> MSEFRIHHDVNELLSLLRVHGGDGAEVYIDLLQKNRTPYVTTTVSAHSAKVKIAEFSRTPEDFLKKYDELKSKNTRNLDPLVYLLSKLTEDKETLQYLQQNAKERAELAAAAVGSSTTSINVPAAASKISMQELEELRKQLGSVATGSTLQQSLELKRKMLRDKQNKKNSGQHLPIFPAWVYERPALIGDFLIGAGISTDTALPIVLLRWNLALSPRLKCSGVISAHCNLHLPGTLPLASQESAVVEDLLYVLVGVDGRYVSAQPLAGRQSRTFLVDPNLDLSIRELVHRILPVAASYSAVTRFIEEKSSFEYGQVNHALAAAMRTLVKEHLILVSQLEQLHRQGLLSLQKLWFYIQPAMRTMDILASLATSVDKGECLGGSTLSLLHDRSFSYTGDSQAQELCLYLTKAASAPYFEVLEKWIYRGIIHDPYSEFMVEEHELRKERIQED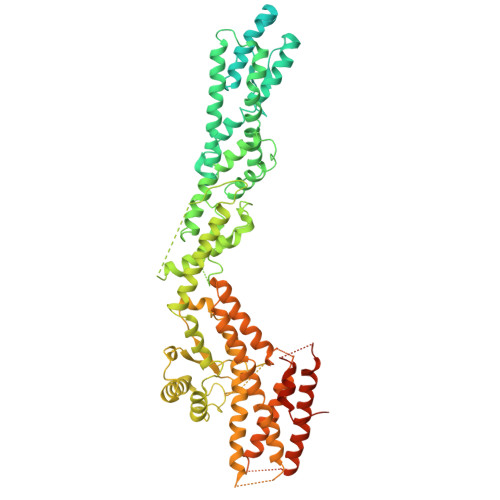YNDKYWDQRYTIVQQQIPSFLQKMADKILSTGKYLNVVRECGHDVTCPVAKEIIYTLKERAYVEQIEKAFNYASKVLLDFLMEEKELVAHLRSIKRYFLMDQGDFFVHFMDLAEEELRKPVEDITPPRLEALLELALRMSTANTDPFKDDLKIDLMPHDLITQLLRVLAIETKQEKAMAHADPTELALSGLEAFSFDYIVKWPLSLIINRKALTRYQMLFRHMFYCKHVERQLCSVWISNKTAKQHSLHSAQWFAGAFTLRQRMLNFVQNIQYYMMFEVMEPTWHILEKNLKSASNIDDVLGHHTGFLDTCLKDCMLTNPELLKVFSKLMSVCVMFTNCMQKFTQSMKLDGELGGQTLEHSTVLGLPAGAEERARKELARKHLAEHADTVQLVSGFEATINKFDKNFSAHLLDLLARLSIYSTSDCEHGMASVISRLDFNGFYTERLERLSAERSQKATPQVPVLRGPPAPAPRVAVTAQ>[3x]MKLPVREFDAVVIGAGGAGMRAALQISQSGQTCALLSKVFPTRSHTVSAQGGITVALGNTHEDNWEWHMYDTVKGSDYIGDQDAIEYMCKTGPEAILELEHMGLPFSRLDDGRIYQRPFGGQSKNFGGEQAARTAAAADRTGHALLHTLYQQNLKNHTTIFSEWYALDLVKNQDGAVVGCTALCIETGEVVYFKARATVLATGGAGRIYQSTTNAHINTGDGVGMAIRAGVPVQDMEMWQFHPTGIAGAGVLVTEGCRGEGGYLLNKHGERFMERYAPNAKDLAGRDVVARSIMIEIREGRGCDGPWGPHAKLKLDHLGKEVLESRLPGILELSRTFAHVDPVKEPIPVIPTCHYMMGGIPTKVTGQALTVNEKGEDVVVPGLFAVGEIACVSVHGANRLGGNSLLDLVVFGRAAGLHLQESIAEQGALRDASESDVEASLDRLNRWNNNRNGEDPVAIRKALQECMQHNFSVFREGDAMAKGLEQLKVIRERLKNARLDDTSSEFNTQRVECLELDNLMETAYATAVSANFRTESRGAHSRFDFPDRDDENWLCHSLYLPESES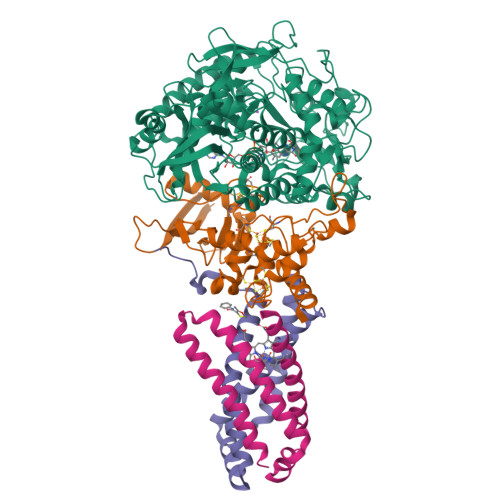MTRRSVNMEPKLRPAFPPKIRTY;>MRLEFSIYRYNPDVDDAPRMQDYTLEADEGRDMMLLDALIQLKEKDPSLSFRRSCREGVCGSDGLNMNGKNGLACITPISALNQPGKKIVIRPLPGLPVIRDLVVDMGQFYAQYEKIKPYLLNNGQNPPAREHLQMPEQREKLDGLYECILCACCSTSCPSFWWNPDKFIGPAGLLAAYRFLIDSRDTETDSRLDGLSDAFSVFRCTSIMNCVSVCPKGLNPTRAIGHIKSMLLQRNA[3x];>[3x]MIRNVKKQRPVNLDLQTIRFPITAIASILHRVSGVITFVAVGILLWLLGTSLSSPEGFEQASAIMGSFFVKFIMWGILTALAYHVVVGIRHMMMDFGYLEETFEAGKRSAKISFVITVVLSLLAGVLVW;>MVSNASALGRNGVHDFILVRATAIVLTLYIIYMVGFFATSGELTYEVWIGFFASAFTKVFTLLALFSILIHAWIGMWQVLTDYVKPLALRLMLQLVIVVALVVYVIYGFVVVWGV[3x]The signal recognition particle (SRP) is an efficient protein sorting system that directs the translocation of newly synthesized proteins from translating ribosomes to the endoplasmic reticulum (ER) or plasma membrane. Similarly, the eukaryotic SRP receptor (SR) consists of two proteins, SRα and the membrane-inserted SRβ, while in bacteria, a single protein, FtsY, is responsible for membrane association and interaction with the translocon. In FtsY, the NG domain (comprising of the N-terminal and GTP binding domains) is involved in binding a GTP molecule and forming a heterodimer with the NG domain of Ffh. The N domain of FtsYNG consists of a four-helix bundle (αN1−N4), while the G domain adopts a classical Ras GTPase fold in which five conserved motifs (G1−G5) are arranged around the nucleotide-binding site.

A 100-molar excess of Fragment 1, 2 or 3 was then added to the drops containing FtsYNG crystals. In the Fo-Fc electron density maps of the holo structures containing Fragment 1, 2 or 3, we observed medium to high densities in the IBD in both copies of FtsYNG. Nevertheless, it is clear that Fragments 1, 2 and 3 bound at two different sites within the IBD in both copies of FtsYNG in the asymmetric unit. The first site is wedged between helix 1 and helix A and involves a stacking with the indole ring of Trp343. The second site is located between helix B and helix 2 and involves a stacking with the aromatic ring of Phe365. Interestingly, the Trp343 site is located between the RNA and GTP-binding sites at the FtsY-Ffh heterodimerization interface whereas the Phe365 site is situated in a hydrophobic patch surrounded by charged residues involved in RNA-binding. While interactions with Trp343 via π-stacking with the core ring structure are observed in the crystal structures with all three fragments, specific interactions with FtsYNG that are unique to each fragment are also observed. In Fragment 1, hydrophobic interactions involving the CγH2 group of Gln339 are also observed whereas in Fragment 2, H-bonds and water bridges with Gly311, Lys312 and Leu340 are seen. Fragment 1 displays hydrophobic interactions with Val403 and H-bonding with Lys406, whereas Fragment 2 forms a water bridge with Gln354 and has hydrophobic interactions with the aliphatic groups of the Lys406 sidechain. The determined KD values between FtsYNG and Fragment 1, Fragment 2 and Fragment 3 are ~100 ± 20, ~100 ± 20 and ~480 ± 20 μM, respectively, while that for GMPPNP is 280 ± 80 μM.

>GFARLKRSLLKTKENLGSGFISLFRGKKIDDDLFEELEEQLLIADVGVETTRKIITNLTEGASRKQLRDAEALYGLLKEEMGEILAKVDEPLNVEGKAPFVILMVGVNGVGKTTTIGKLARQFEQQGKSVMLAAGDTFRAAAVEQLQVWGQRNNIPVIAQHTGADSASVIFDAIQAAKARNIDVLIADTAGRLQNKSHLMEELKKIVRVMKKLDVEAPHEVMLTIDASTGQNAVSQAKLFHEAVGLTGITLTKLDGTAKGGVIFSVADQFGIPIRYIGVGERIEDLRPFKADDFIEALFARED[2x]>[2x]MAHHHHHHVTNSTDGRADGRL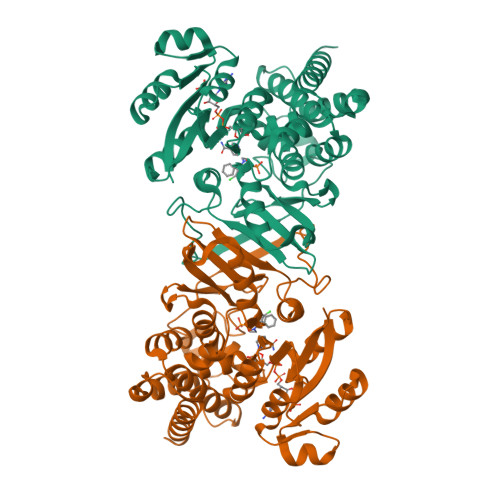RVVVLGSTGSIGTQALQVIADNPDRFEVVGLAAGGAHLDTLLRQRAQTGVTNIAVADEHAAQRVGDIPYHGSDAATRLVEQTEADVVLNALVGALGLRPTLAALKTGARLALANKESLVAGGSLVLRAARPGQIVPVDSEHSALAQCLRGGTPDEVAKLVLTASGGPFRGWSAADLEHVTPEQAGAHPTWSMGPMNTLNSASLVNKGLEVIETHLLFGIPYDRIDVVVHPQSIIHSMVTFIDGSTIAQASPPDMKLPISLALGWPRRVSGAAAACDFHTASSWEFEPLDTDVFPAVELARQAGVAGGCMTAVYNAANEEAAAAFLAGRIGFPAIVGIIADVLHAADQWAVEPATVDDVLDAQRWARERAQRAVSGM>[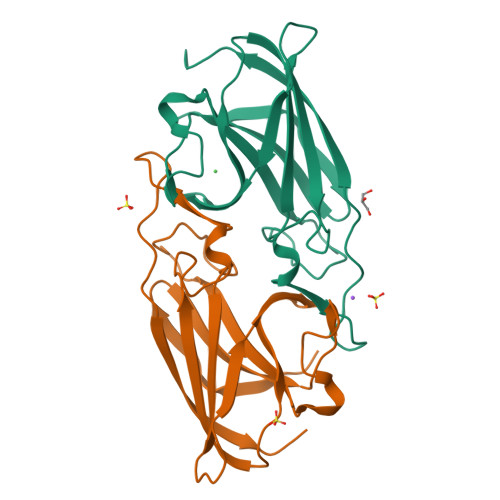2x]MLEYPIGTPQNLAGMEIAAVYLQPIDMEPEGHMRKASESDIHIEADIHALSNNPNGYPEGFWVPFLFIKYEITKVGGSGAPITGDMMAMVASDGPHYGDNVKLQGPGKYKVKYTIYPPNAKENPMSPYYGRHTDRETGVRPWFKTFSVEWDFTYAGIGKKGGYAAALEHHHHHH6-[4-[[3-oxidanyl-1,1-bis(oxidanylidene)-5-phenyl-2-propan-2-yl-3~{H}-1,2-thiazol-4-yl]amino]butyl]pyridine-2-sulfonamide | C21 H28 N4 O5 S2 | 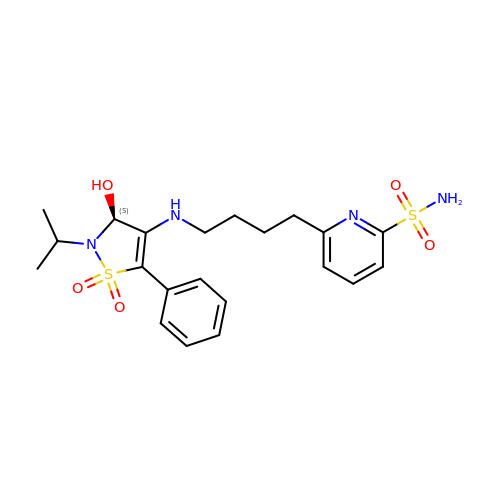VNMXCAMPCSTLPS-NRFANRHFSA-N To neutralize chemokines, ticks secrete small cysteine-rich chemokine-binding proteins in their saliva with no homologues in mammals, termed Evasins. In contrast to the highly selective Evasin-1, its homologue Evasin-4 binds ∼20 CC-chemokines with nanomolar affinity. Among this broad range of chemokines, the chemokine CC-motif ligand 5 (CCL5, also known as RANTES) is of particular interest, because it is one of the most expressed chemokines by activated platelets and plays a prominent role in the development of atherosclerosis. Thus, Evasin-4 binds to the CCL5 monomer and causes disruption of the CCL5 dimer by shifting the monomer/dimer equilibrium toward the monomeric form of the chemokine and not by direct replacing of CCL5 from the dimer.

CCL5 can oligomerize, forming dimers and oligomers of a higher order, which would complicate analysis of Evasin-4 binding. To prevent higher-order CCL5-oligomerization, the E66S CCL5 mutant was used for further experiments, as it mainly forms dimers at physiological pH. Unfortunately, several trials to crystallize Evasin-4 in complex with E66S CCL5 were unsuccessful, primarily because of the precipitation of the complex in solution, even at a low concentration. Although solubility was improved to some extent by increasing the amount of salt in the protein buffer or adding organic solvents such as glycerol, crystals that were obtained in these trials consisted of E66S CCL5 only. These crystals were used to solve the E66S CCL5 structure by X-ray crystallography. As expected, E66S CCL5 formed a dimer and had a structure very similar to that of WT CCL5 with a root-mean-square deviation (RMSD) of 0.63 Å for the backbone of the full-length protein. This confirmed that the E66S mutation disturbed neither the CCL5 folding nor the formation of a dimer. The chemical perturbation plot of monomer/dimer equilibria obtained from the 15N-1H HSQC spectrum of 20 μm E66S CCL5 at pH 4.5, showed that dimerization mostly affected residues of the N-terminal region (Ser4–Ile15), 30s loop (Ser31–Cys34), and β3-strand (Arg47–Cys50). This observation goes in line with the obtained crystal structure because the E66S CCL5 dimer interface is formed by interactions of the N terminus with the 30s loop and β3-strand. The affected residues comprised a continuous surface in the 3D structure of E66S CCL5, coinciding with the E66S CCL5 dimer interface, which suggests that binding of Evasin-4 causes disruption of the CCL5 dimer.

>[2x]SPYSSDTTPCCFAYIARPLPRAHIKEYFYTSGKCSNPAVVFVTRKNRQVCANPEKKWVREYINSLSMS> MRVTVSIIKADVGGFPGHAHVHPKMLEYAAAKLKEAQKRGVIIDYFVYNVGD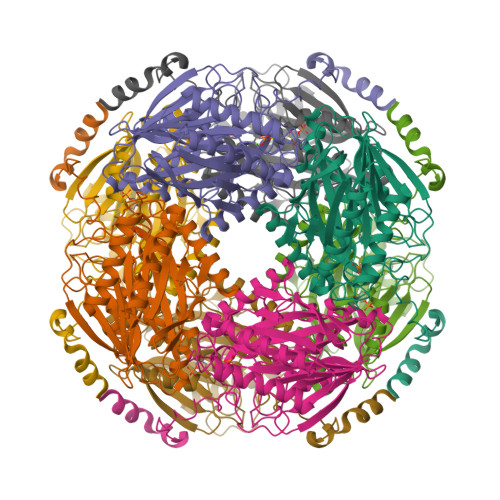DISLLMTHTKGEDNKDIHGLAWETFKEVTDQIAKRFKLYGAGQDLLKDAFSGNIRGMGPQVAEMEFEERPSEPIIAFAADKTEPGAFNLPLYKMFADPFTTAGLVIDPSMHEGFIFEVLDVVEHKVYLLKTPEDAYSLLGLIGTTGRYIIRKVFRRADGAPAAANSVERLSLIAGRFVGKDDPVLLVRAQSGLPAVGEVLEAFAHPHLVHGWMRGSHAGPLMPARFISVDPERRIAIGPKMTRFDGPPKVGALGFQLHEGYLEGGVDLFDDPAFDYVRQTAAQIADYIRRMGPFQPHRLPPEEMEYTALPKILAKVKPYPADQYEKDRKKYIEAVVKGAKVEESQHDLEHHHHHH>[2x]MPEEKELLELLEELENIFSRSPSD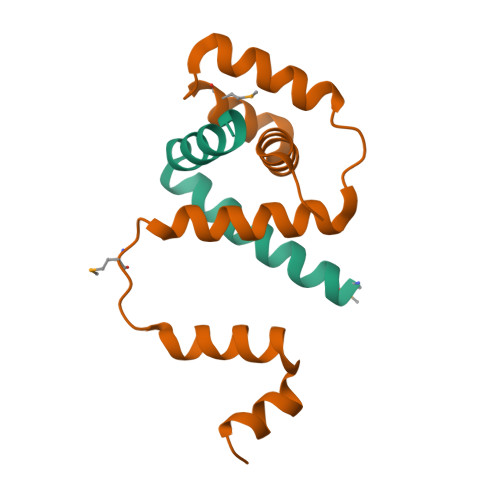IAEIVRLWFFERGLENLYF;>MPEKKIDGRRKAAVLLVALGPEKAAQVMKHLDEETVEQLVVEIANIGRVTPEEKKQVLEEFLSLAKAKEMISEGGIEYAKKVLEKAFGPERARKIIER[2x]> SLIV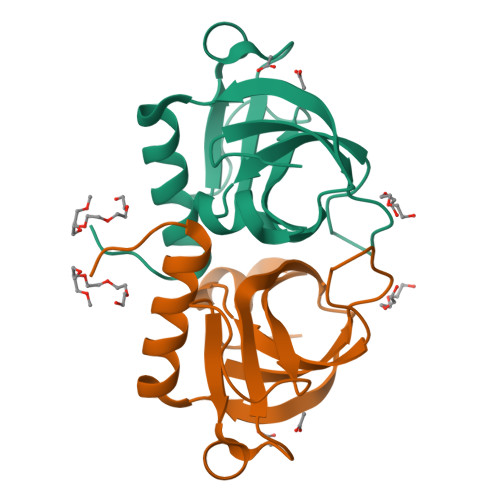KRGDVYFADLSPVVGSEQGGVRPVLVIQNDIGNRFSPTAIVAAITAQIQKAKLPTHVEIDAKRYGFERDSVILLEQIRTIDKQRLTDKITHLDDEMMDKVDEALQISLALIDF(3R)-3-[3-(4-chlorophenyl)-1,2,4-oxadiazol-5-yl]piperidine | C13 H14 Cl N3 O | 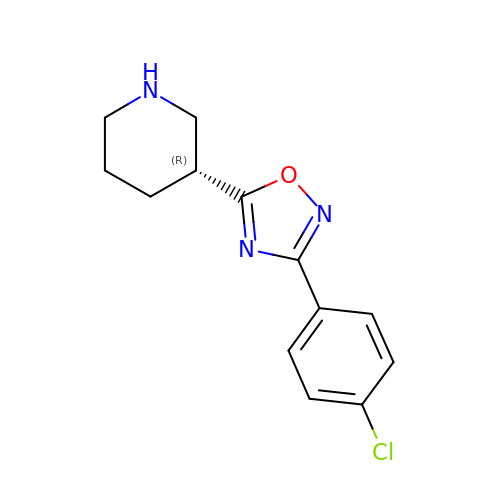ROGHUOMPUVCGAA-SNVBAGLBSA-N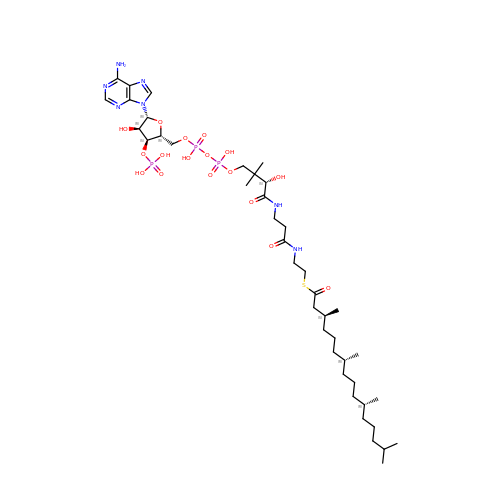S-{(3R,5S,9S)-1-[(2R,3S,4R,5R)-5-(6-amino-9H-purin-9-yl)-4-hydroxy-3-(phosphonooxy)oxolan-2-yl]-3,5,9-trihydroxy-8,8-dimethyl-3,5,10,14-tetraoxo-2,4,6-trioxa-11,15-diaza-3lambda~5~,5lambda~5~-diphosphaheptadecan-17-yl} (3S,7R,11R)-3,7,11,15-tetramethylhexadecanethioate (non-preferred name) | C41 H74 N7 O17 P3 S | NRJQGHHZMSOUEN-KBMDNNSFSA-N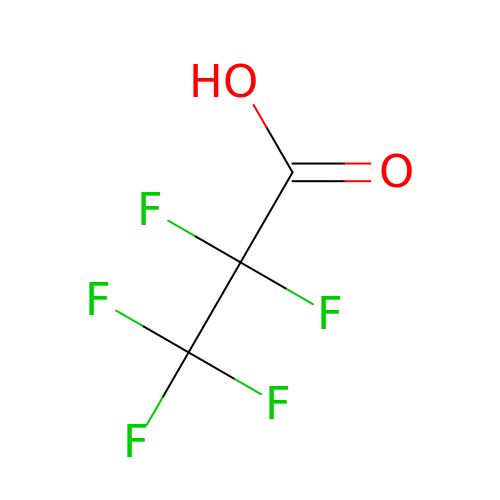pentafluoropropanoic acid | C3 H F5 O2 | LRMSQVBRUNSOJL-UHFFFAOYSA-N>SHRYVETMLVADQSMAEFHGSGLKHYLLTLFSVAARLYKHPSIRNSVSLVVVKILVIHDEQKGPEVTSNAALTLRNFCNWQKQHNPPSDRDAEHYDTAILFTRQDLCGSQTCDTLGMADVGTVCDPSRSCSVIEDDGLQAAFTTAHELGHVFNMPHDDAKQCASLNGVNQDSHMMASMLSNLDHSQPWSPCSAYMITSFLDNGHGECLMDKPQNPIQLPGDLPGTSYDANRQCQFTFGEDSKHCPDAAST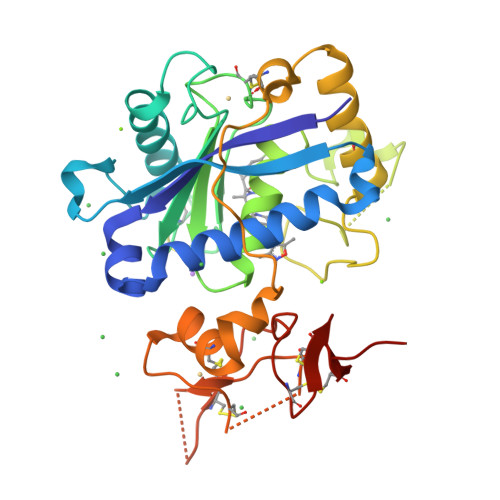CSTLWCTGTSGGVLVCQTKHFPWADGTSCGEGKWCINGKCVNKLVPR[2x]>[2x]GVEPQVGIVNGLAVYGPNSGSLLEIEVSVTAAQDKGSINITGIAEEESIGSQSKSIRRKSMAKGSVENVLTVLRTMGMKPSDYDIHINFPGGIPIDGPSAG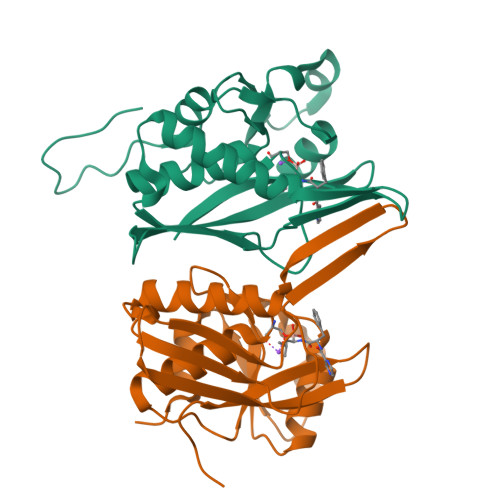IAMAAGIFSAIHKIPIDNTVAMTGEISLNGLVKPIGGVIPKIKAAKQSGAKKVIIPYENQQAILKQIDGIEIIAVKTFQEVLDEILVNPPTEQKPFHIEINKESV>[2x]MVGQIAKEMGLRAYIVGGVVRDILLGKEVWDVDFVVEGNAIELAKELARRHGVNVHPFPEFGTAHLKIGKL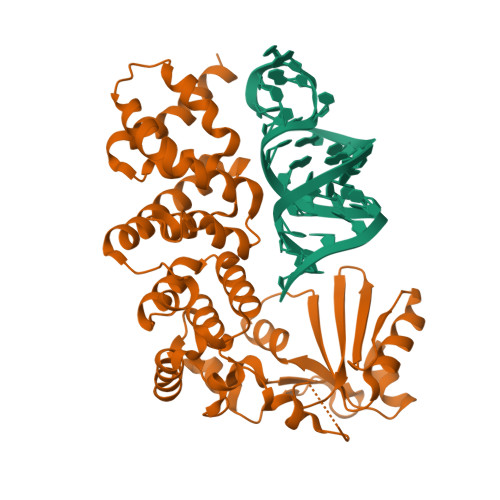KLEFATARRETYPRPGAYPKVEPASLKEDLIRRDFTINAMAISVNLEDYGTLIDYFGGLRDLKDKVIRVLHPVSFIEDPVRILRALRFAGRLNFKLSRSTEKLLKQAVNLGLLKEAPRGRLINEIKLALREDRFLEILELYRKYRVLEEIIEGFQWNEKVLQKLYALRKVVDWHALEFSEERIDYGWLYLLILISNLDYERGKHFLEEMSAPSWVRETYKFMKFKLGSLKEELKKAKENYEVYRLLKPLHTSVLLLLMLEEELKEKIKLYLEKLRKVKLPKEKIEELKKQGLKGKELGERIEELKREIMNKIKLAAALE>SNAMGLDVRNNGNDNVEIRAAETRTAQRADEALETAADFAGQPKVTHTMRTINRTLSRRISRNTGSEQVLNLRRLMEKYLEDTRFKDDFIFVAVDPNQYSVPYPTLVVMSGAKVGDHNHFFGYVLPLVAGLAPLPRREEQGPHGNILVPRTWVDNLNGTFINEVMAAMYAAIGGKSNGTARIAGLAVVTNEITAESAHLATTLLSAADNAIQTAIEIRLGDKLGLPQFNLGMMASDQPISSVQYNTSGMQDSDIVGNPVRSDITVTISNRIRQAMSDYDSQQRLVATTGYIDLTYSPQNPTFNQGPVLVNGYPVPPTVQYQPRYVMTSAYPLELDAFTPNTFVLGLIGTIATLNSGMAWAQSLISNAARGIGPHNPGALAMVLDPEVTAPLDLSTQTNEQIYKFLQQVLYPSLLISIDVPEEGEYSWLLRMIPAAEKIYTGKVEGEVREISEGYKALYRAFDDVTLGCFSKKYQYGLPLVYATGNRIPLGHYNHQDGHRHDIRDMDDLYMMNITNPDTVEAWEDSFDRTDMTMSQRVVARHEIIDRVLSGSWEQTGWAMRYDFDPLALQALIEAAADAGFTIRPENIQHLAGTAVRGNMAARARGLGNISGNIYARSDRPNVGVNNMGGAFNLF[4x]

In response, one family of large bacteriophages uses a nucleus-like compartment to protect its replicating genomes by excluding host defence factors. Here we find that the bacteriophage nuclear shell assembles primarily from one protein, which we name chimallin (ChmA). Combining cryo-electron tomography of nuclear shells in bacteriophage-infected cells and cryo-electron microscopy of a minimal chimallin compartment in vitro, we show that chimallin self-assembles as a flexible sheet into closed micrometre-scale compartments. We find that the shell is primarily composed of a single protein, chimallin, which self-assembles through its extended N and C termini into a closed compartment.

We obtained a 4.2 Å-resolution structure of the overall Goslar chimallin assembly, and used a similar localized reconstruction procedure as for the 201phi2-1 chimallin to obtain a 2.6 Å-resolution structure of the Goslar chimallin tetramer, and a 2.3 Å-resolution structure of a single protomer. Overall, Goslar chimallin shows high structural homology to 201phi2-1 chimallin despite the low overall sequence identity, with a Cɑ r.m.s.d. of 1.8 Å within a protomer and 4.8 Å over an entire C4-symmetric tetramer. The NTS, CTS1 and CTS2 segments of Goslar chimallin show near-identical interactions to neighbouring protomers compared with 201phi2-1 chimallin with the exception of CTS2, which is shorter in Goslar than in 201phi2-1 and shows a distinct set of interactions. Thus, together with our findings on 201phi2-1 and Goslar, these data show that despite extremely low sequence conservation, chimallin proteins from divergent jumbo phages exhibit high structural conservation at both the level of an individual protomer and overall nuclear shell architecture.> MAGVSAVSKVSSLVCDLSSTSGLIRRTANPHPNVWGYDLVHSLKSPYIDSSYRERAEVLVSEIKAMLNPAITGDGESMITPSAYDTAWVARVPAIDGSARPQFPQTVDWILKNQLKDGSWGIQSHFLLSDRLLATLSCVLVLLKWNVGDLQVEQGIEFIKSNLELVKDETDQDSLVTDFEIIFPSLLREAQSLRLGLPYDLPYIHLLQTKRQERLAKLSREEIYAVPSPLLYSLEGIQDIVEWERIMEVQSQDGSFLSSPASTACVFMHTGDAKCLEFLNSVMIKFGNFVPCLYPVDLLERLLIVDNIVRLGIYRHFEKEIKEALDYVYRHWNERGIGWGRLNPIADLETTALGFRLLRLHRYNVSPAIFDNFKDANGKFICSTGQFNKDVASMLNLYRASQLAFPGENILDEAKSFATKYLREALEKSETSSAWNNKQNLSQEIKYALKTSWHASVPRVEAKRYCQVYRPDYARIAKCVYKLPYVNNEKFLELGKLDFNIIQSIHQEEMKNVTSWFRDSGLPLFTFARERPLEFYFLVAAGTYEPQYAKCRFLFTKVACLQTVLDDMYDTYGTLDELKLFTEAVRRWDLSFTENLPDYMKLCYQIYYDIVHEVAWEAEKEQGRELVSFFRKGWEDYLLGYYEEAEWLAAEYVPTLDEYIKNGITSIGQRILLLSGVLIMDGQLLSQEALEKVDYPGRR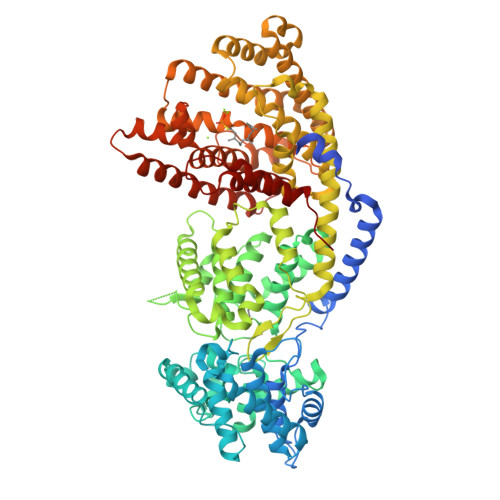VLTELNSLISRLADDTKTYKAEKARGELASSIECYMKDHPECTEEEALDHIYSILEPAVKELTREFLKPDDVPFACKKMLFEETRVTMVIFKDGDGFGVSKLEVKDHIKECLIEPLPL> GAMQQTFASKTEWRTRAIATSNLRTRANNMYVAPVDNDVDDITYVMPKNILKKFITIADLRVQVAGFLYGCSPADNDQVKEIRCIVMVPQIGGNRSVQLPQHLPQHE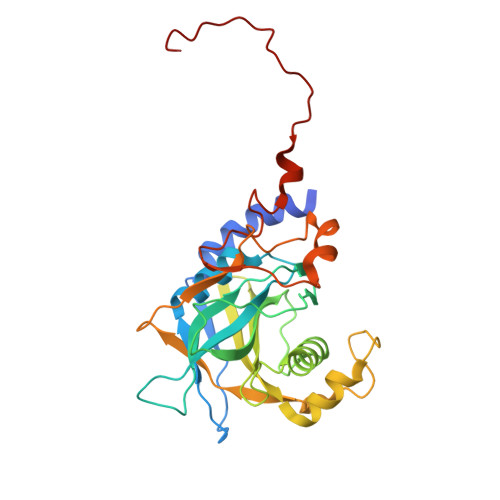MLKGLEPLGLIHTMAGNELPYMSPADVTTHAKLVDAHPSWKNQNTLTVTVAFTPGSVSLSAWALTPLGYKWGVENKDPNVDNPQGFTTTMGERRQLLLSDKFKGFFLVPDTGKWNYSFMGSSFSGIEKKPYHVKLDTPLPFYSEQHRPIHFTSFNELEDIWVDRADNFA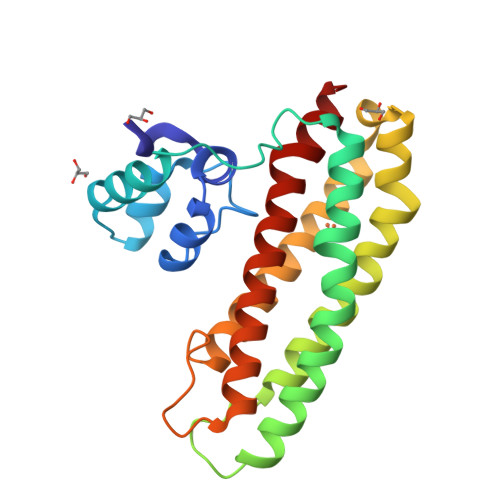>[2x]AYRDQPLGELALSIPRASALFRKYDMDYAAGGKQTLARAAARKELDVEVIEAELAKLAEQPIEKDWRSAPLAEIIDHIIVRYHDRHREQLPELILQATKVERVHADKPSVPKGLTKYLTMLHELLSSHMMKEEQILFPMIKQGMGSQAMGPISVMESEHDEAGELLEVIKHTTNNVTPPPEACTTWKAMYNGINELIDDLMDHISLENNVLFPRALAGE> GPGSVPELKQISR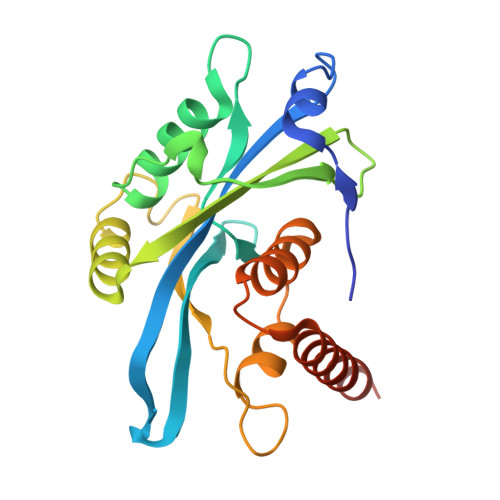VEAMRLGPGWSHSCHAMLYAANPGQLFGRIPMRFSVLMQMRFDGLLGFPGGFVDRRFWSLEDGLNRVLGLGLGCLRLTEADYLSSHLTEGPHRVVAHLYARQLTLEQLHAVEISAVHSRDHGLEVLGLVRVPLYTQKDRVGGFPNFLSNAFVSTAKCQLLFALKVLNMMPEEKLVEALAAATEKQKKALEKLLPASS In pacidamycin 3, biosynthesis the 3′‐deoxy moiety is mediated by Pac13, an enzyme found to catalyze the key dehydration of uridine‐5′‐aldehyde 1 to form 3′‐deoxy‐3′,4′‐didehydrouridine‐5′‐aldehyde 2. In stark contrast to most characterised dehydratases, Pac13 is small (121 aa), monomeric, co‐factor independent and utilises a non‐activated nucleoside, rather than a free monosaccharide, as a substrate. Pac13 is the only monomeric, metal‐free cupin dehydratase characterised to date. We demonstrate here that the reaction most likely proceeds via an E1Cb mechanism, with H42 acting as an active site base, however, unlike many other dehydratases, no metal or cofactor is required for activity.

Initial soaks with uridine‐5′‐aldehyde 1, the natural substrate, were problematic due to both turnover and the inherent instability of this molecule. In order to overcome this problem we used substrate analogues, uridine 7 and uridine 5′‐uronic acid 8, which enabled us to obtain liganded complexes of the enzyme, providing the first clues of the location and structural determinants of the active site. Both ligands occupied the same binding pocket in their respective co‐crystal structures. Comparison of the apo‐ and ligand‐bound structures revealed that small movements in residues such as K16, F103 and L21 create a pocket that encloses the ribose ring of the substrate analogues but leave one side of the uracil group solvent exposed. Within the ribose pocket, the 5′ oxygen lies almost equidistant (2.5–2.7 Å) between Y55 and Y89, with a slightly shorter distance to Y89, whereas the 4′ proton and 3′ hydroxy are 2.7–3 Å from H42. In contrast to this extensive network of direct polar interactions the uracil ring makes a single H‐bond to K16 at the lip of the active site, with more Van der Waals (L21, V34, V99) and π‐stacking interactions (F103) characterising recognition of this part of the substrate. Notably, lipophilic residues L97 and V36 border the active site, creating a hydrophobic environment and perhaps sheltering the substrate or dehydrated product from attack from water. An E1cB mechanism can be postulated from the structure to be likely: in the first step, H42 could act as base extracting the activated 4′ proton, creating an enolate 10. The oxyanion could then be stabilised by hydrogen bonding by Y55 and Y89, and the protonated H42 could then act as the acid, donating a proton to 3′ hydroxy group of the substrate and thus generating a better leaving group.

> GSHMTKYKYTVEESERFNKHGIDLTVYGQVDPSATVVRVSVERGHFQEFFNVRSSYTYYVVSGQGVFYLNSEAVPAGATDLITVPPNTRIHYFGSMEMVLTVAPAFNEQDERHVRFISESESPY>[2x]GFCWHHS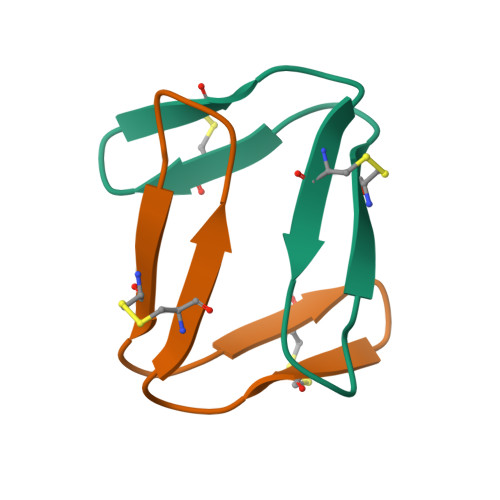CVPSGTCADFPWPLGHQCFPD> MTSRKKVLLKVIILGDSGVGKNSLMNQYVNKKFSNQYKATIGADFLTKEVMVDDRLVTMQIWDTAGQERFQSLGVAFYRGADCCVLVFDVTAPNTFKTLDSWRDEFLIQASPRDPENFPFVVLGNKIDLENRQVATKRAQAWCYSKNNIPYFETSAKEAINVEQAFQTIARNALKQET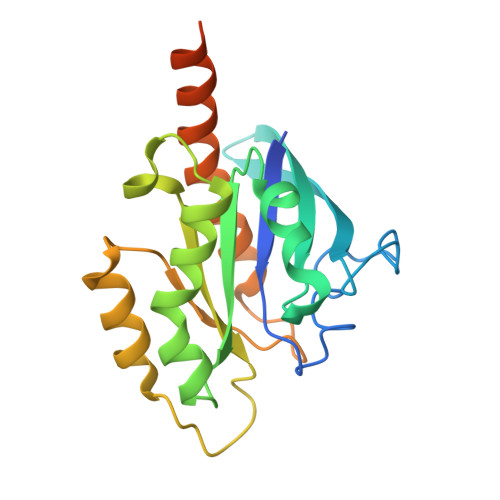EVELYNEFPEPIKLDKNDRAKASAESCSC>IISRNFPIIGVKEKTFEQLHKKCLEKKVLYVDPEFPPDETSLFYSQKFPIQFVWKRPPEICENPRFIIDGANRTDICQGELGDSWFLAAIACLTLNQHLLFRVIPHDQSFIENYAGIFHFQFWRYGEWVDVVIDDCLPTYNNQLVFTKSNHRNEFWSALLEKAYAKLHGSYEALKGGNTTEAMEDFTGGVAEFFEIRDAPSDMYKIMKKAIERGSLMGCSIDDGTNMTYGTSPSGLNMGELIARMVRNMDNSLLQDSDLDPRGSDERPTRTIIPVQYETRMACGLVRGHAYSVTGLDEVPFKGEKVKLVRLRNPWGQVEWNGSWSDRW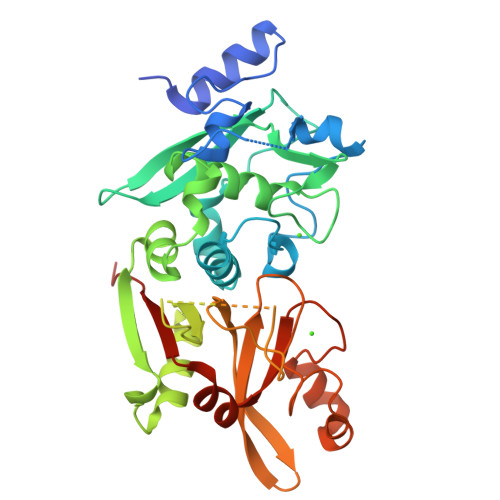KDWSFVDKDEKARLQHQVTEDGEFWMSYEDFIYHFTKLEICNLTADLEHHHHHH[4x]>VSNAIKFIILTEIIFPTLLLVFGIYHGVMQVFYRSGIIKAESFLGIDYYQGLTLHGVINVIVYTTIFIVGFSNAIVAYSLKKPLREKVQWIALGMMVIGTLMAAWAMFTGRATVLYTFYPPLIAHWTFYLGAVLLVLGSLVPFFFDWIPSAIQWKRENPDQKLPLAVFGTFVNFILWTIMIVPVAIEILFQLLPLSLGLVDEINPLLARTLFWFFGHPVVYFWLLPAYVALYTILPKIVSEKGKLYSDPAARLAFILFLIFSLPVGLHHQFTDPGITNTWKLIHALFTFGVALPSMITAFTVATSLEYSVKAEHPELKNSKFYWWTFLPFMRLEGNKWMFSYFFAGLVLFFIGGITGIVNASYNVNLVVHNTAYVPGHFHTTVGGLVLLVFFALSLYMVSKLRGSEVKLKGLAVLAPYFWMQGMFMFSYAMMVGGVVVGFPRRTNAGLTYLNPDSPLYRPEWTGYAQLAAVGGVLLAIGFAFYFASLIATALAPKVRESTLEFPIADAYHDAPAPLLNNLKTWTVAAIILAVLSYIPPLYDASVRGVFFKSPAYNEKFPMPLKQLQGAEKKEEKKELSKAEGGITQK[2x];>[2x]RAEKTGLTLALILLLTFFSLIVYAAKGLKIDIPTCVTDVEPFQEGKLIKHGDKRYELHILARMWYFDFNKGATEIKIPVGSVVDIFTTSKDVVHGVHIHGTNYNVMAIPGTVGYMRIKFEKPGVYHVVCHEFCGVGHHAMQGKIIVE;>[2x]FFPSGTIAFFIFMMVFYAVLWFMIYWVLLERG

Cytochrome c oxidase (CcO) is the terminal enzyme in the respiratory chains of many aerobic organisms. It is located in the inner membrane of mitochondria and bacteria, and catalyzes the electron transfer from cytochrome c to molecular oxygen that is reduced to water. The cytochrome c oxidase from A. aeolicus, AaCcO, was previously discovered belonging to B‐family HCO, and interestingly could use both cytochrome c and ubiquinol as electron donors, which is a unique feature as a member of B‐family HCO. To gain insights into the molecular mechanism of AaCcO and also to understand how AaCcO adapts its structure to keep stability and activity under hyperthermophilic growth conditions, we purified the AaCcO from native membranes and determined its structure at 3.4 Å resolution by using single‐particle electron cryo‐microscopy (cryo‐EM).

We found a dimeric form of AaCcO with a novel binding site of the native quinol (VII‐tetrahydromultiprenyl‐1,4 naphthoquinone, NQ) at the dimeric interface, which could allow NQH2 to be a direct electron donor bypassing cytochrome c. Surprisingly, subunit I (CoxA2) contains 14 TMHs, two more than the canonical structures of CcOs. The AaCcO dimer is formed via interactions of its major subunit CoxA2 while this is not the case for BtCcO. Interestingly, two quinol molecules (NQ) are found at the interface with the head group orientation towards the P‐side. Each NQ molecule is deeply buried in the hydrophobic groove formed by subunits IIa and coxA2. In particular, one carbonyl oxygen of NQ is found to bind to Glu39 of subunit IIa, a residue presents only in A. aeolicus. To be noted, the NQ tail is buried inside one protomer while its carbonyl oxygen is proximal to heme b of another protomer. The edge‐to‐edge distance between NQ and heme b is 15.0 Å. Thus, only the K‐pathway does exist for proton transfer in AaCcO. However, structural superposition of AaCcO and TtCcO suggest that only one oxygen diffusion channel exists and forms a V‐shape in AaCcO.>QDSLSFGFPTFPSDQKNL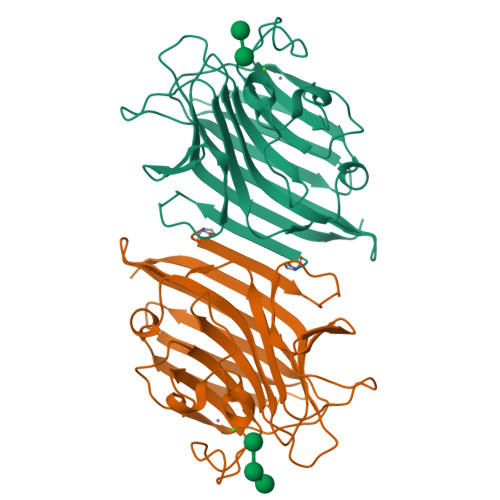IFQGDAQIKNNAVQLTKTDSNGNPVASTVGRILFSAQVHLWEKSSSRVANFQSQFSFSLKSPLSNGADGIAFFIAPPDTTIPSGSGGGLLGLFAPGTAQNTSANQVIAVEFDTFYAQDSNTWDPNYPHIGIDVNSIRSVKTVKWDRRDGQSLNVLVTFNPSTRNLDVVATYSDGTRYEVSYEVDVRSVLPEWVRVGFSAASGEQYQTHTLESWSFTSTLLYTAQKKGENLALEM[2x]OCP is a water-soluble, carotenoid-binding, 35 kDa protein found to induce dissipation of phycobilisome excitation energy minimizing energy flux toward the reaction centers. Unlike the wide variety of HCPs, the CTD homologs (CTDH) fall only into two clades, of which only one is present in Anabaena (a clade 2 CTDH). Recently, it was revealed that isolated CTD of Synechocystis OCP and CTDHs from Anabaena and Thermosynechococcus elongatus (a clade 1 CTDH) are also capable of carotenoid binding. Both CTD and CTDH were shown to mediate carotenoid transfer to apo-OCP, apo-NTD, or apo-HCP (from clade 4). Thus one likely role of CTDHs is to serve as intermediate transfer molecules required for delivery of carotenoids from membranes to the HCPs.

In order to obtain a more homogeneous preparation of apo-AnaCTDH dimers, we added 2 M urea to the solution, which caused a large proportion of the high oligomeric states to disassemble, resulting in predominantly dimeric CTDH (solid line). Crystals were obtained in the presence of urea. The asymmetric unit dimer (hence called A-type or back-to-back) was formed via an interaction plane between the β-sheets of two monomers, quite distant from Cys103. PISA suggested that only the F-type dimer has biological significance, (ΔiGP value of 0.067 for the F-type dimer interface). The presence of the disulfide bond forces the formation of the F-type dimer of apo-AnaCTDH. The most striking difference between the apo-AnaCTDH structure presented here and the CTD-OCPO structure is a major shift in the position of the C-terminal tail. In contrast, in the apo-AnaCTDH structure, the C-terminal tail adopts an internal position, coming closer to the F-type interface between the CTDH monomers (CTD-NTD interface in OCP), partially covering the opening of the designated carotenoid-accommodating cavity in the apo-AnaCTDH structure. Owing to the steric constraints, the F-type crystallographic apo-AnaCTDH dimer is not capable of performing carotenoid uptake from the membranes, as the carotenoid channel is partially blocked by the C-terminal tail and filled with the Cys103-containing loop (hereafter β5/β6 loop), while in the A-type dimer, the carotenoid cavity is open. Thus the F-type dimer cannot accommodate the carotenoid unless structural changes occur.

>SIAGITEPTILQYFATLNAGEFAATAALFAVDGVMYPPFESGIVGPDAIAAYLQQEAQGIKAEPQQGLAETSEDGHTQVQVSGKAQTSWCGVNVLWLFTLNQEKQIIHTQIKLLASPQELLALR[2x]DNA polymerase theta (Polθ) has been identified as a crucial alternative non-homologous end-joining factor in mammalian cells. Polθ is distinct among human DNA polymerases, exhibiting not only a C-terminal DNA polymerase domain (Seki et al., 2003, Shima et al., 2003, Yousefzadeh and Wood, 2013) but also an N-terminal domain exhibiting similarity and motifs typical of superfamily 2 (SF2) helicases (Singleton et al., 2007), separated by a long and lesser-conserved central domain of unknown function (Seki et al., 2003, Shima et al., 2003, Yousefzadeh and Wood, 2013) (Singleton et al., 2007). The Polθ helicase domain (Polθ-HLD) is a member of the SF2 helicases, most closely related to the Ski2/Hel308 family of helicases, which are involved in the ATP-dependent 3′-5′ unwinding of lagging strands on replication forks (Tafel et al., 2011, Buttner et al., 2007, Guy and Bolt, 2005), thought to facilitate replication restart at stalled or damaged forks. Like its archaeal homologs, Polθ-HLD comprises five subdomains including the two core helicase domains and three additional, closely associated globular domains.

We determined the structure of Polθ-HLD (residues 67–894), in a complex with the non-hydrolysable ATP analogue AMP-PNP to 2.9-Å resolution, and with ADP to 3.2-Å resolution, both in the same crystal form with a single copy of Polθ-HLD in the asymmetric unit. In the nucleotide-bound complexes, AMP-PNP and ADP bind in the nucleotide-binding site in a similar conformation to that observed in other helicase complexes. The adenine moiety is hydrogen bonded to the conserved glutamate of the helicase motif 0 or “Q motif,” although in Polθ-HLD the adenine moiety stacks against V89 and F93 rather than the conserved Leu and Arg residues common to the RecQ family. The α, β, and γ phosphates are in the equivalent positions as found in other helicase nucleotide complexes with conserved polar contacts formed to resides in the helicase motif I. The electron density for the AMP-PNP molecule is significantly weaker than in the ADP complex, especially around the adenine and ribose moieties, suggesting only partial occupancy in these crystals. Comparing the relative orientations of the D1 and D2 domains in the apo and nucleotide-bound Polθ-HLD crystals reveals a modest difference in relative domain orientation (maximal displacements of up to 5 Å), which would place the ssDNA-binding motifs slightly closer together in the nucleotide-bound crystals. Analysis of the nucleotide-bound crystals reveals that the same arrangement can be formed from the crystallographic symmetry operators, suggesting the tetramer is unlikely to be a result of crystal packing interactions. Comparing these profiles directly with theoretical scattering profiles calculated from the Polθ-HLD tetramer crystal structure reveals good agreement between the experimental profiles and the Polθ-HLD tetramer in crystals (χ2 = 1.60, χ2 free = 1.80).

> SMDKLLLANWGLPKAVLEKYHSFGVKKMFEWQAECLLLGQVLEGKNLVYSAPTSAGKTLVAELLILKRVLEMRKKALFILPFVSVAKEKKYYLQSLFQEVGIKVDGYMGSTSPSRHFSSLDIAVCTIERANGLINRLIEENKMDLLGMVVVDELHMLGDSHRGYLLELLLTKICYITRKSASCQADLASSLSNAVQIVGMSATLPNLELVASWLNAELYHTDFRPVPLLESVKVGNSIYDSSMKLVREFEPMLQVKGDEDHVVSLCYETICDNHSVLLFCPSKKWCEKLADIIAREFYNLHHQAEGLVKPSECPPVILEQKELLEVMDQLRRLPSGLDSVLQKTVPWGVAFHHAGLTFEERDIIEGAFRQGLIRVLAATSTLSSGVNLPARRVIIRTPIFGGRPLDILTYKQMVGRAGRKGVDTVGESILICKNSEKSKGIALLQGSLKPVRSCLQRREGEEVTGSMIRAILEIIVGGVASTSQDMHTYAACTFLAASMKEGKQGIQRNQESVQLGAIEACVMWLLENEFIQSTEASDGTEGKVYHPTHLGSATLSSSLSPADTLDIFADLQRAMKGFVLENDLHILYLVTPMFEDWTTIDWYRFFCLWEKLPTSMKRVAELVGVEEGFLARCVKGKVVARTERQHRQMAIHKRFFTSLVLLDLISEVPLREINQKYGCNRGQIQSLQQSAAVYAGMITVFSNRLGWHNMELLLSQFQKRLTFGIQRELCDLVRVSLLNAQRARVLYASGFHTVADLARANIVEVEVILKNAVPFKSARKAVDEEEEAVEERRNMRTIWVTGRKGLTEREAAALIVEEARMILQQDLVEM>[2x]MSHWLMKSEPESRLEKGVDVKFSIEDLKAQPKQTTCWDGVRNYQARNFLRAMKLGEEAFFY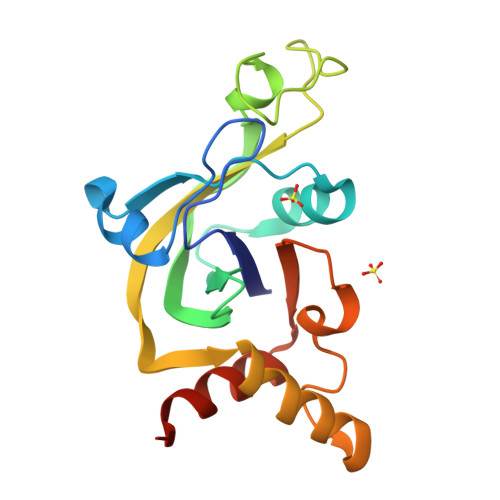HSNCKEPGIAGLMKIVKEAYPDHTQFEKNNPHYDPSSKEDNPKWSMVDVQFVRMMKRFIPLAELKSYHQAHKATGGPLKNMVLFTRQRLSIQPLTQEEFDFVLSLEELEHHHHHH> DSMYGFIGTDVVLHCSFANPLPGVKITQVTWQKATNGSKQNVAIYN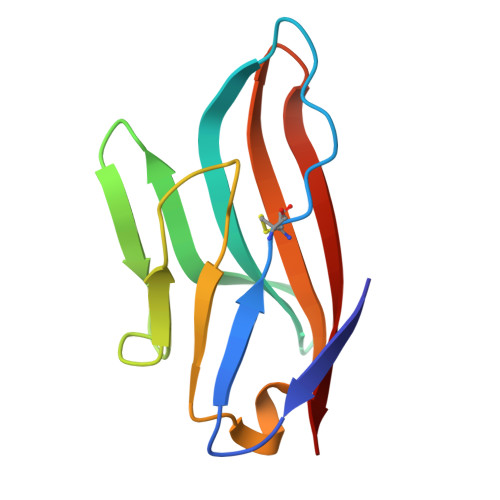PAMGVSVLAPYRERVEFLRPSFTDGTIRLSRLELEDEGVYICEFATFPAGNRESQLNLTVM> ANPLYQKHIISINDLSRDDLNLVLATAAKLKANPQPELLKHKVIASCFFEASTRTRLSFETSMHRLGASVVGFSDSANTSLGKKGETLADTISVISTYVD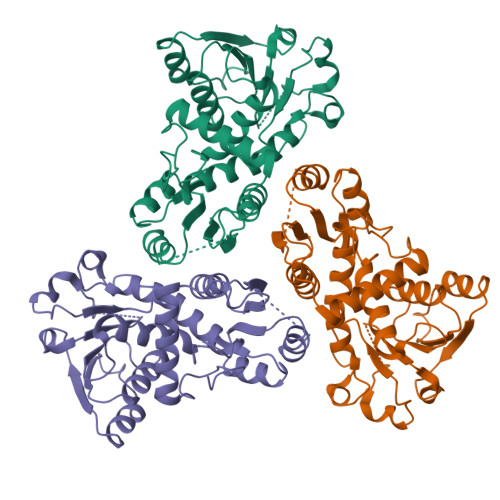AIVMRHPQEGAARLATEFSGNVPVLNAGDGSNQHPTQTLLDLFTIQETQGRLDNLHVAMVGDLKYPRTVHSLTQALAKFDGNRFYFIAPDALAMPQYILDMLDEKGIAWSLHSSIEEVMAEVDILYMTRVQKERLDPSEYANVKAQFVLRASDLHNAKANMKVLHPLPRVDEIATDVDKTPHAWYFQQAGNGIFARQALLALVLNRDLVL(2E,2'E)-3,3'-(1,2-phenylene)di(prop-2-enoic acid) | C12 H10 O4 | 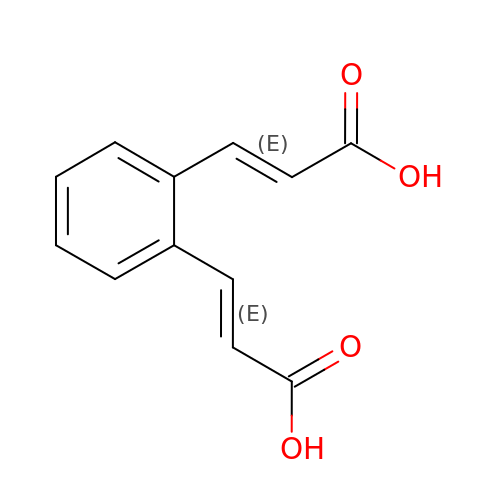ZFCNOKDRWHSHNR-KQQUZDAGSA-N S-HYDROPEROXYCYSTEINE | C3 H7 N O4 S | 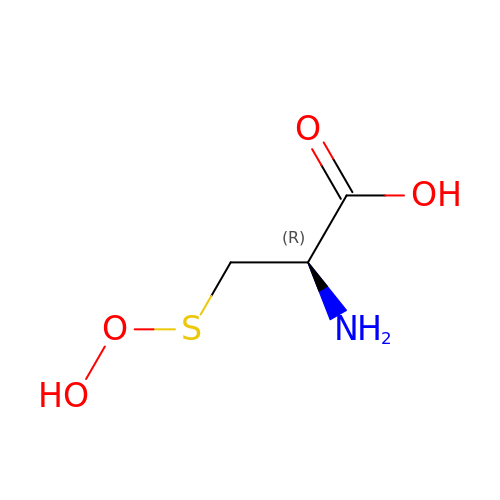BXTMIEGCNKHUKA-REOHCLBHSA-N>MVFLPLKWSLATMSFLLSSLLALLTVSTPSWCQSTEASPKRSDGTPFPWNKIRLPEYVIPVHYDLLIHAQLTTLTFWGTTKVEITASQPTSTIILHSHHLQISRATLRKGAGERLSEEPLQVLEHPRQEQIALLAPEPLLVGLPYTVVIHYAGQLSETFHGFYKSTYRTKEGELRILASTQFEPTAARMAFPCFDEPAFKASFSIKIRREPRHLAISNMPLVKSVTVAEGLIEDHFDVTVKMSTYLVAFIISDFESVSKITKSGVKVSVYAVPDKINQADYALDAAVTLLEFYEDYFSIPYPLPKQDLAAIPDFQSGAMENWGLTTYRESALLFDAEKSSASSKLGITMTVAHELAHQWFGNLVTMEWWNDLWLNEGFAKFMEFVSVSVTHPELKVGDYFFGKCFDAMEVDALQSSHPVSTPVENPAQIREMFDDVSYDKGACILNMLREYLSADAFKSGIVQYLQKHSYKNTKNEDLWDSMASIGSGGVDVKTMMNTWTLQKGFPLITITVRGRNVHMKQEHYMKGSDGAPDTGYLWHVPLTFITSKSDMVHRFLLKTKTDVLILPEEVEWIKFNVGMNGYYIVHYEDDGWDSLTGLLKGTHTAVSSNDRASLINNAFQLVSIGKLSIEKALDLSLYLKHETEIMPVFQGLNELIPMYKLMEKRDMNEVETQFKAFLIRLLRDLIDKQTWTDEGSVSERMLRSQLLLLACVHNYQPCVQRAEGYFRKWKESNGQLSLPVDVTLAVFAVGAQSTEGWDFLYSKYQFSLSSTEKSQIEFALCRTQNKEKLQWLLDESFKGDKIKTQEFPQILTLIGRNPVGYPLAWQFLRKNWNKLVQKFELGSSSIAHMVMGTTNQFSTRTRLEEVKGFFSSLKENGSQLRCVQQTIETIEENIGWMDKNFDKIRVWLQSEKLERMENLYFQ[2x]

Endoplasmic reticulum aminopeptidase 1 (ERAP1) cleaves the N-terminal amino acids of peptides, which can then bind onto major histocompatibility class I (MHC-I) molecules for presentation onto the cell surface, driving the activation of adaptive immune responses. Given that ERAP1-trimmed peptides modulate the adaptive immune response, controlling ERAP1 activity is an attractive strategy for cancer immunotherapy, autoimmune diseases and increasing immune responses against pathogens. Herein we describe the hit-to-lead optimization of a series of cyclohexyl acid ERAP1 inhibitors, found by X-ray crystallography to bind at an allosteric regulatory site. Binding of peptides to the regulatory site plays a critical role in determining ERAP1 substrate length requirements and the extent to which peptide trimming occurs through a “molecular ruler” mechanism.

Also discovered in the same high-throughput screen as the clerodane acid derivative was the hit cyclohexyl acid compound 1, which had ERAP1 inhibitory potency and a selectivity profile similar to those of the clerodane acid derivative. Hit compound 1 was found by X-ray crystallography to bind at the same regulatory site as the clerodane acid derivative. In this assay, compound 1 had an ERAP1 pIC50 value of 5.5. Three major binding interactions were observed from the carboxylic acid of compound 1 to Arg807, Lys685 and Tyr684. These key interactions are thought to be where the C-termini of endogenous peptides bind. The cyclohexane ring occupied a lipophilic pocket, and the attached amide did not clearly show any specific polar interactions with the protein. An additional hydrogen bond interaction was observed from the carbonyl of the thiomorpholinone motif with Gln881. Adjacent to the aromatic ring of the benzothiomorpholinone was a pocket containing lipophilic residues Phe674 and Leu677, shown to be occupied by a water molecule. The first area investigated was the substitution of the bicyclic motif, as the X-ray cocrystal structure indicated potential space for growth into the lipophilic pocket containing Phe674 and Leu677. Compound 1 had reduced structural complexity compared to the clerodane acid derivative and was therefore considered a more synthetically tractable molecule for hit-to-lead optimization.>SREDLRAWLTRNRFPRVGGVSESTVQWEGVVFTVSNESVPRWVMAQIQPAYMGLVATQASLAAAEAVAAVARRRGIEVHGPLQVADPNDPAASRSQVALLLSELRRAGCREIAVDLTGGKLPMSLGAFMAAEEAGVA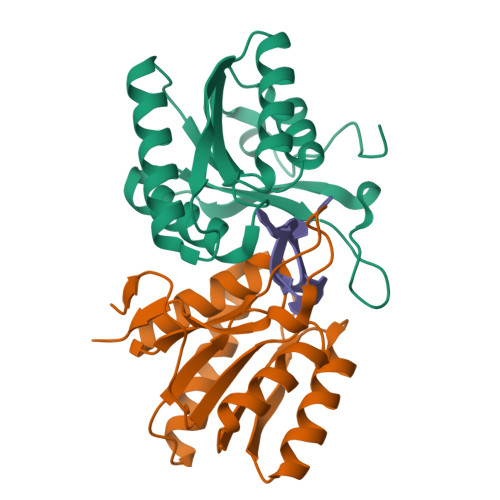SLYVATDFDKHLKVPDMRTATLRQISQPE[2x]> MTDDKDVLRDVWFGRIPTCFTLYQDEITEREAEPYYLLLPRVSYLTLVT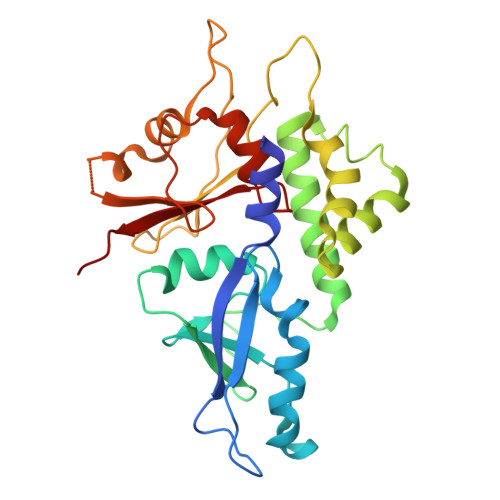DKVKKHFQKVMRQEDISEIWFEYEGTPLKWHYPIGLLFDLLASSSALPWNITVHFKSFPEKDLLHCPSKDAIEAHFMSCMKEADALKHKSQVINEMQKKDHKQLWMGLQNDRFDQFWAINRKLMEYPAEENGFRYIPFRIYQTTTERPFIQKLFRPVAADGQLHTLGDLLKEVCPSAIDPEDGEKKNQVMIHGIEPMLETPLQWLSEHLSYPDNFLHISIIPQPTD> MGQSHTHDHHHDGYQAPPEDIALRVKALESLLIEKGLVDPAAMDLVV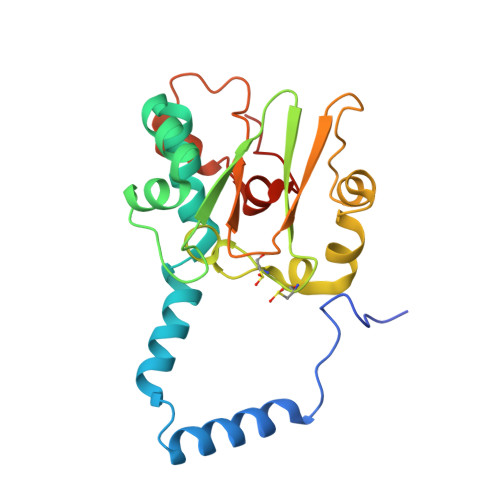QTYEHKVGPRNGAKVVAKAWVDPAYKARLLADGTAGIAELGFSGVQGEDMVILENTPAVHNVFVCTLCSCYPWPTLGLPPAWYKAAPYRSRMVSDPRGVLAEFGLVIPANKEIRVWDTTAQLRYMVLPERPAGTEAYSEEQLAELVTRDSMIGTGLPTQPTPSH> SQCSSTLVKHIKAPLHLVWSIVRRFDEPQKYKPFISRCVVQGKKLEVGSVREVDLKSGLPATKSTEVLEILDDNEHILGIRIVGGDHRLKNYS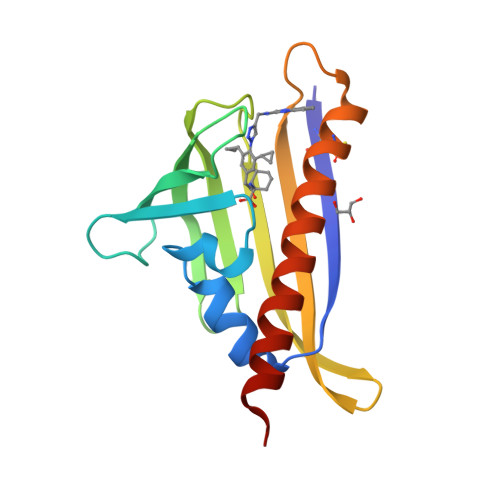STISLHSETIDGKTGTLAIESFVVDVPEGNTKEETCFFVEALIQCNLNSLADVTERLQAESMEKKI>SNAMTERKIFNRLKSVLAEKGKTNLWLTETLDKNKTTVSKWCTNDVQPSLETLFDIAEALNVDVREL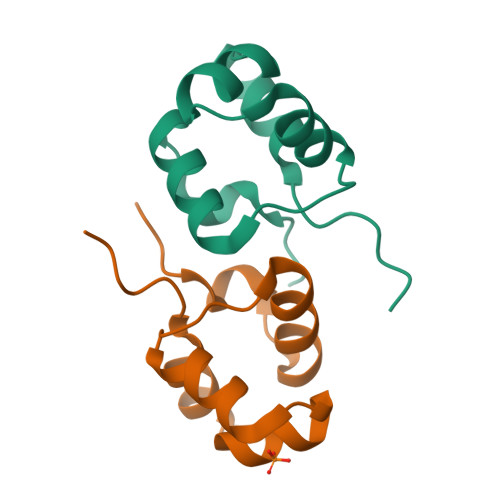IVSTKR[2x]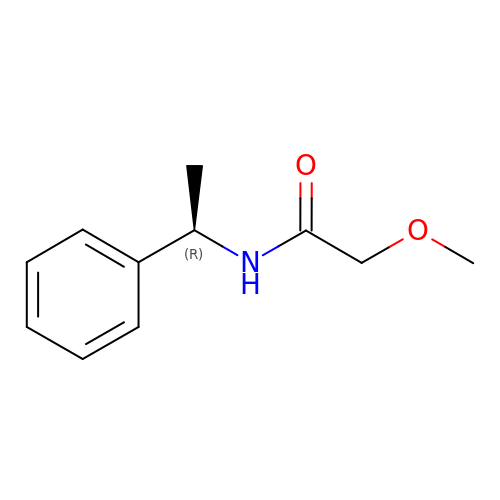2-methoxy-N-[(1R)-1-phenylethyl]acetamide | C11 H15 N O2 | LJEDIKNIRTZHGK-SECBINFHSA-N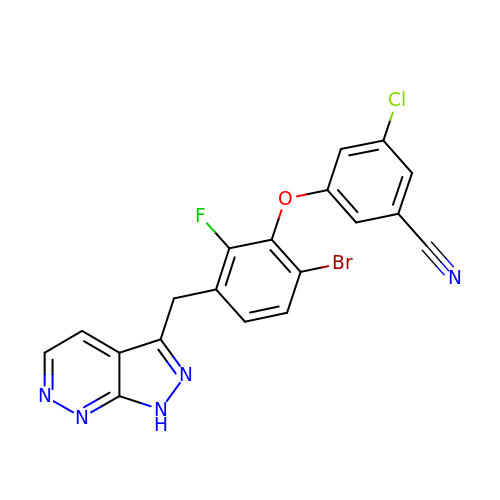3-[6-bromo-2-fluoro-3-(1H-pyrazolo[3,4-c]pyridazin-3-ylmethyl)phenoxy]-5-chlorobenzonitrile | C19 H10 Br Cl F N5 O | OHQMEDBYNUAVNE-UHFFFAOYSA-N> MNKPVISRAEQIFYPGWLMVSQLRSGQPVEDGKALYRRACQLVKQAREE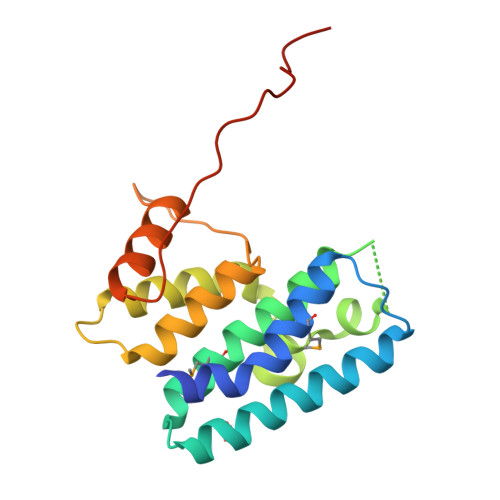LAEAGFSQKSSDIMLYAFCALLDESVLNREKTDDGWRTWQQDPLQAHFFGTLNAGEELWERIREQLKLPAPDVAVLTCLCRTLQLGFTGQYRSQDDERREDVIRALTARVPAFTFAQDAPVVVRAPGYRAGRTM>HHHHHHELMTDKTLQQIDKLICSWLKQIDNVIPQLIMEMTTETKRHRFDLVTNVDKQIQQQFQQFLATYFPEHQLLAEEKSNAMITNEINHLWIMDPIDGTANLVKQQEDYCIILAYFYEGKPMLSYVYDYPHKKLYKAIRGEGAFCNGIKMEEPPSLKLEDAIISFNAQVMNLDTVQDLFDASFSYRLVGACGLDSMRVAKGQFGAHINTNPKPWDIAAQFLFAELLNLKMTTLDGKAIDHLKGAPFIISNKACHETVLKIL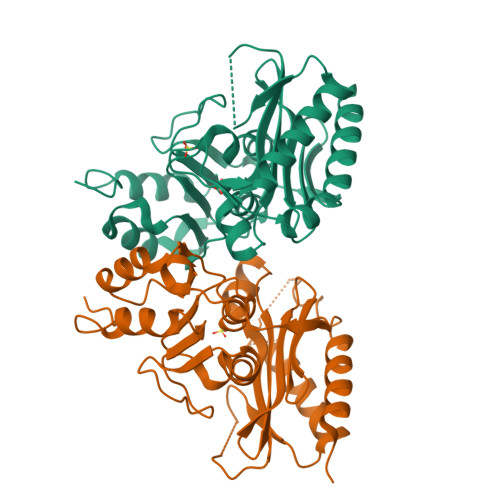NANGGYQKYR[2x]> MRSNKRQIIEKAIERKNEIETLPFDQNLAQLSKLNLKGETKTKYDAMKKDNVESTNKYLAPVEEKIHNAEALLDKFSFNASQSEIDDANELMDSYEQSYQQQLEDVNEIIALYKDNDELYDKCKVDYREMKRDVLANRHQFGEAASLLETEIEKFEPRLEQYEVLKADGNYVQAHNHIAALNEQMKQLRSYMHGSSGN

By contrast, the integral membrane protein EzrA was identified as an inhibitor of FtsZ polymerization and its absence results in the inappropriate formation of multiple FtsZ rings, not only at mid-cell but also at the cell poles. EzrA comprises a single, N-terminal trans-membrane (TM) spanning helix followed by an ~60-kDa cytoplasmic domain15, which sequence analysis suggests forms an α-helical coiled-coil. The BsEzrA22–562 and the shorter SaEzrA24–214 rods comprise multiple copies of the same ~100 amino acid, triple helical bundle; BsEzrA22–562 contains five such repeats and SaEzrA24–214 contains just two. Although many proteins are known to comprise bundles of antiparallel α-helices, EzrA is, to the best of our knowledge, the only bacterial protein that is formed from serial spectrin-like repeats.

To obtain higher resolution structural information on EzrA, several fragments from different EzrA homologues were subjected to crystallization. A 190 residue N-terminal fragment of S. aureus EzrA, SaEzrA24–214 (that also lacks its N-terminal TM helix), yielded crystals that diffracted to 2.6 Å resolution. Its structure was solved by molecular replacement using model phases from the equivalent portion of BsEzrA22–562, and was refined to a final crystallographic Rfree of 0.25. The structures of SaEzrA24–214 and BsEzrA22–562, which share only 20% sequence identity, superpose with root mean square deviations (RMSDs) of 2.4 Å on 154 paired Cα atoms. Two copies of the spectrin repeats are also observed in a 2.6-Å resolution structure of a 20-kDa cytoplasmic fragment of EzrA from S. aureus (Sa), which has enabled direct molecular comparisons to be made between eukaryotic spectrin repeats and those found in EzrA. As also observed in several spectrins, the SaEzrA24–214 structure reveals intimate interactions at the interface between repeats involving the linker helix and loop residues. For example, the linker residues Tyr135 and Ile131 interact with loop residues Thr62, Leu56 and Tyr193. The angle between the two repeats in SaEzrA24–214 is 34°, suggesting that full-length EzrA from S. aureus will also have a pronounced bend. The first and third repeats in EzrA each contain a highly conserved proline residue in helix A; Pro45 of SaEzrA in repeat 1 is conserved in eight out of nine phylogenetically diverse paralogues, whereas Pro228 (Pro227 in BsEzrA) in repeat 3 is conserved in all of them. The conserved proline in helix 1 of repeat 1 (Pro45 in S. aureus EzrA) may confer some additional flexibility in the junction between the body of the cytoplasmic domain and the membrane.> MKVAVLVGGVGRRIGMEKTEVMLCGKKLIEWVLEKYSPFQTVFVCRDEKQAEKLSSRYEAEFIWDLHKGVGSIAGIHAALRHFGSCVVAAIDMPFVKPEVLEHLYKEGEKAGCDALIPKHDYPEPLLAYYAESAADELERAILQG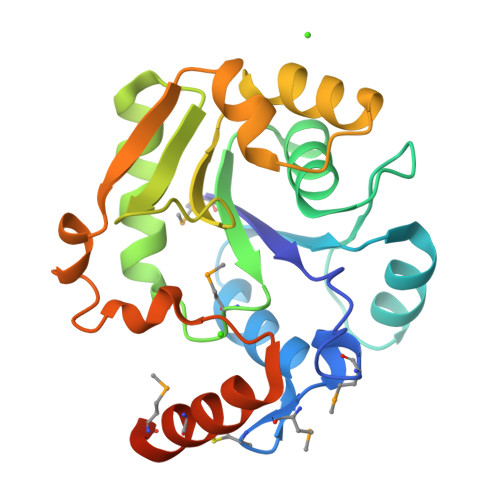IRKILVPLERLNVVYYPVEKLRKFDKELISFFNINTPDDLKRAEEICSKMSTEGLLEHHHHHH>[2x]GSAMARKRIITPEKKELIRNLISEYNITSAKDLQEALKDLLGDTIQNMLEAELDEHLGYEKYESTEEAKSNYRNGYTSKTLKSSVGQVEIDIPRDRNAEFEPKIVPRYKRDISEIENKIIAMYARGMSTREINEQIQEIYGFEVSAEMVSKITDKILPEIEEWQKRPLGEVYPIVFIDAIHFSVKNDGIVGKKAVYIVLAIDIEGQKDVIGIYVGENESSKFWLSV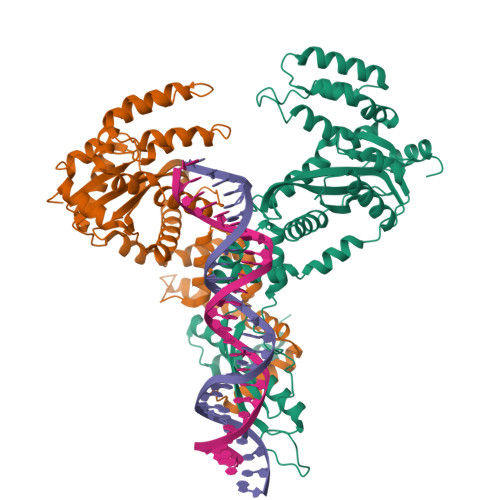LNDLKNRGVKDILILCADALSGIKDAINAAFPNTEYQRCIVHQIRNTLKYVSDKDRKEFARDLKRIYTAPNEKAGYDQMLEVSEKWEKKYPAAMKSWKSNWDVICPFFKYSEELRKIMYTTNTIESLNSSYRRINKSRTVFPGDQSLLKSIYLATVKITSKWTMRYKNWGLILGQLQIMFEGRI Hexameric MCM rings act as the replicative DNA helicase, encircling the leading strand DNA template at the replication fork. Mcm2-7 complexes are loaded to encircle double-stranded DNA (dsDNA) via a ‘gate’ between Mcm2 and Mcm5 to yield a double hexamer that does not unwind DNA. During helicase activation, the Dbf4-dependent Cdc7 kinase (DDK) and cyclin-dependent kinases (CDKs) drive recruitment of Cdc45 and the GINS complex. These factors stimulate the Mcm2-7 ATPase and helicase and with Mcm2-7 form the CMG complex (Cdc45-Mcm2-7-GINS), the active replicative helicase. Following activation, two Mcm2-7 helicases encircle single-stranded DNA (ssDNA) and translocate independently, 3ʹ→5ʹ, on the leading strand DNA template with the ATPase domain leading.

We identified a chimera of the N-terminal domain of Sulfolobus solfataricus (Sso) and the AAA+ domain of PfMCM, Sso-PfMCM with a robust DNA unwinding activity. The N-terminal domain of SsoMCM (residues 1–269, top sequence) was fused to the AAA+ domain of PfMCM (starting at residue 257, bottom sequence) to yield the chimera (middle sequence). The Sso-PfMCM hexamer forms a ring with a channel large enough to accommodate double-stranded DNA (dsDNA) (see ‘Materials and methods’). The two-tiered structure is consistent with electron microscopy studies. The N-terminal tier has three subdomains, A–C with the A-subdomains in a different orientation (see below) than observed previously. The A-subdomains of Sso-PfMCM are rotated 150° compared to those in SsoMCMN. In Sso-PfMCM, the change correlates with a conformer change in P104 at the junction of the A/C-subdomains (phi/psi = −48.5/133.0 in Sso-PfMCM vs −78.0/−14.9 in SsoMCMN, Liu et al., 2008). The h2i creates a DNA-binding pocket at the MSSB where ssDNA was observed previously. In each subunit of our Sso-PfMCM hexamer crystal structure, residues 198–212 comprise a conserved loop of the OB-fold that projects towards the h2i of the same subunit and the ps1β of an adjacent subunit. The structure reveals a fully conserved glutamine, Q198, of the ACL interacts with the main-chain amide atoms of the h2i. The ATPase active site structurally resembles the ATPase site of the AAA+ helicase E1 (2:04) with Walker-A/B residues of one subunit, and three positively charged residues of the adjacent subunit.

>SLEIPSKQIDYRDVFIEFLTTFKGNNNQNKYIERINELVAYRKKSLIIEFSDVLSFNENLAYEIINNTKIILPILEGALYDHILQLDPTYQRDIEKVHVRIVGIPRVIELRKIRSTDIGKLITIDGILVKVTPVKERIYKATYKHIHPDCMQEFEWPEDEEMPEVLEMPTICPKCGKPGQFRLIPEKTKLIDWQKAVIQERPEEVPSGQLPRQLEIILEDDLVDSARPGDRVKVTGILDIKQDSPVKRGSRAVFDIYMKVSSIEVSQKVLQELEISPEEEQIIKELAKRKDIVDAIVDSIAPAIYGYKEVKKGIALALFGGVSRKLPDGTRLRGDIHVLLVGDPGVAKSQILRYVANLAPRAIYTSGKSSSAAGLTAAAVRDEFTGGWVLEAGALVLADGGYALIDELDKMSDRDRSVIHEALEQQTISISKAGITATLNARTTVIAAANPKQGRFNRMKNPFEQIDLPPTLLSRFDLIFVLIDEPDDKIDSEVARHILRVRRGESEVVAPKIPHEILRKYIAYARKNIHPVISEEAMEEIEKYYVRMRKSVKKTKGEEEGIPPIPITARQLEALIRLSEAHARMRLSPIVTREDAREAIKLMEYTLKQIAMD[2x]> MANGYTYEDYQDTAKWLLSHTEQRPQVAVICGSGLGGLVNKLTQAQTFDYSEIPNFPESTVPGHAGRLVFGILNGRACVMMQGRFHMYEGYPFWKVTFPVRVFRLLGVETLVVTNAAGGLNPNFEVGDIMLIRDHINLPGFSGENPLRGPNEERFGVRFPAMSDAYDRDMRQKAHSTWKQMGEQRELQEGTYVMLGGPNFETVAECRLLRNLGADAVGMSTVP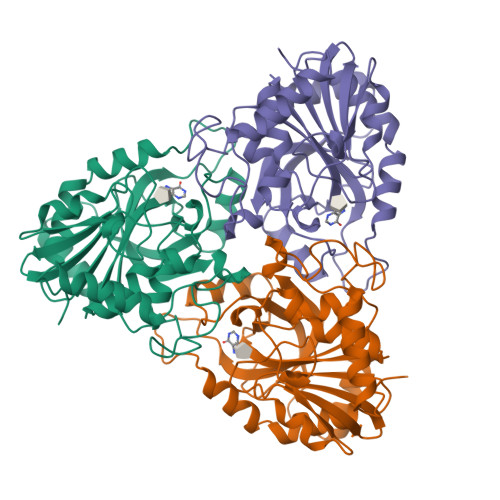EVIVARHCGLRVFGFSLITNKVIMDTESQGKANHEEVLEAGKQAAQKLEQFVSLLMASIPV> MKTQVAIIGAGPSGLLLGQLLHKAGIDNVILERRTPDYVLGRIRAGVLEQGMVDLLREAGVDRRMARDGLVHEGVEIAFAGQRRRIDLKR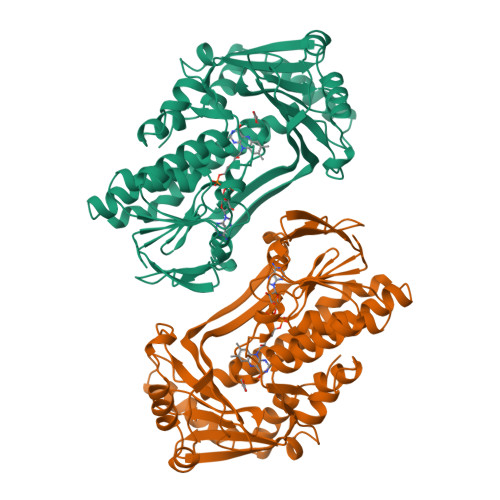LSGGKTVTVYGQTEVTRDLMEAREASGATTVYQAAEVRLHDLQGERPYVTFERDGERLRLDCDYIAGCDGFHGISRQSIPAERLKVFERVYPFGWLGLLADTPPVSHELIYANHPRGFALCSQRSATRSRYYVQVPLTEKVEDWSDERFWTELKARLPAEVAEKLVTGPSLEKSIAPLRSFVVEPMQHGRLFLAGDAAHIVPPTGAKGLNLAASDVSTLYRLLLKAYREGRGELLERYSAICLRRIWKAERFSWWMTSVLHRFPDTDAFSQRIQQTELEYYLGSEAGLATIAENYVGLPYE> MTSPLDPHSKCYSHINGSAEELLDRL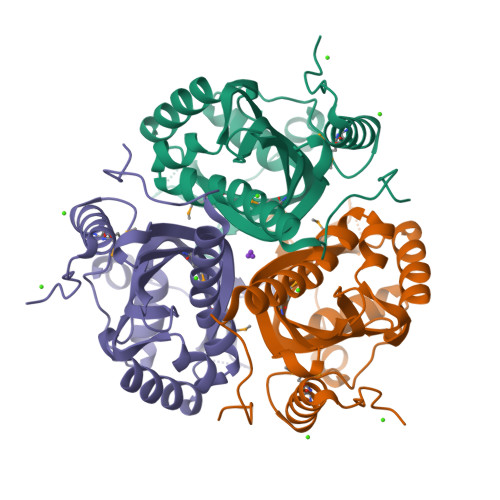AVSELCKGWPVYRDASEWKNYRSLFTEDATVWTTWSGPRPVDEFITISKAGKEQGVFIMHRECGTLVELSPQQGRAIGKMKATITQRFSFPAASGAATNGTTGTTSDAIEFDVDCDCRFIFFCEKDTASGAWKAKYVKLFYEKDKVVSVDGHQAPKFTKDELAKYPQGYRYLGAAQARLGYDIDLQLPTSSGQLWDRMYGEMENWLGGNKVDLFWEH>[2x]GPLGSPEFPGRLEDVTVYSLEDLTALASEHTSKNTDTFAAVFSFLSGRLVHISEQAALILNSKRGFLKSVHFVDLLAPQDVRAFYAHTAPTQLPFWNNWTQRASQYECAPAKPFFCRICGGGDREKRHYSPFRILP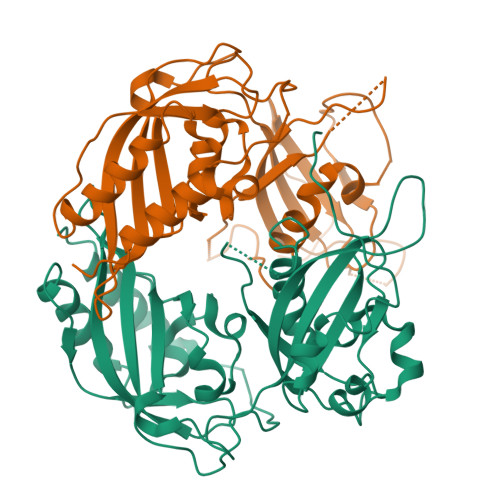YLVHVHSSAQPEPEPCCLTLVEKIHSGYEAPRIPVDKRIFTTTHTPGCVFLEVDERAVPLLGYLPQDLIGTSILTYLHPEDRPLMVAIHQKVLKYAGHPPFEHSPVRFCTQNGEYVILDSSWSSFVNPWSRKVSFIIGRHKVRTSPLNEDVFATRIKKAASNDKDIAELQEQIHKLLLQPV>[6x]KKARMTVDKDY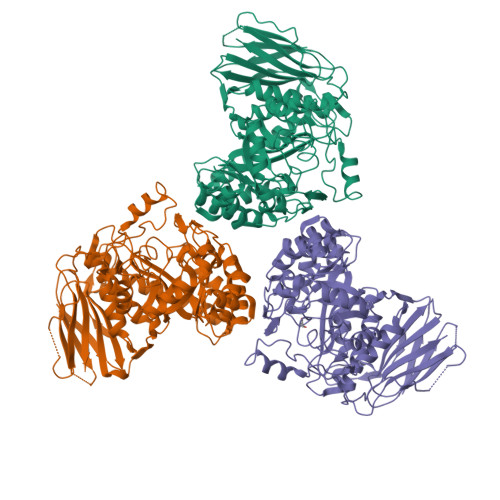KIAEIDKRIYGSFVEHLGRAVYDGLYQPGNSKSDEDGFRKDVIELVKELNVPIIAYPGGNFVSNYFWEDGVGPVEDRPRRLDLAWKSIEPNQVGINEFAKWCKKVNAEIMMAVNLGTRGISDACNLLEYCNHPGGSKYSDMRIKHGVKEPHNIKVWCLGNEMDGPWQVGHKTMDEYGRIAEETARAMKMIDPSIELVACGSSSKDMPTFPQWEATVLDYAYDYVDYISLHQYYGNKENDTADFLAKSDDLDDFIRSVIATCDYIKAKKRSKKDIYLSFDEWNVWYHSNNEDANIMQNEPWRIAPPLLEDIYTFEDALLVGLMLITLMKHADRIKIACLAQLINVIAPIVTERNGGAAWRQTIFYPFMHASKYGRGIVLQPVINSPLHDTSKHEDVTDIESVAIYNEEKEEVTIFAVNRNIHEDIVLVSDVRGMKDYRLLEHIVLEHQDLKIRNSVNGEEVYPKNSDKSSFDDGILTSMLRRASWNVIRIG> HHHHHHHHSQAGDTLNDVIQDPTRRNKLINDNNLLKGIIMGRDGPVPSSRELIVRPDTLRAIINNRATIETTTMEAEFTETLMESNYNSASVKVSAPFITANSEYSESSSFKNTETEKSMYTSSRYLFPQGRIDFTTPDSGFDDVIKLSPQFTSGVQAALAKATGTEKREALQNLFQEYGHVFRTKVHIGGVLSAHTMETFSRSENETEVKQDVKAGLEGAVKGWGGGATAGHGNTQGTITTSQNRKLNVKYIVNGGDYTKIQNTEEWVASTNQSEHWRVIEVT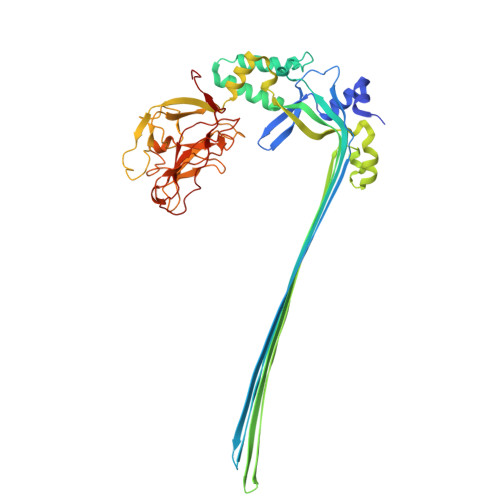EVTAVADLLPQPIRGQVKDLLKPLLGKWVDVEKVPGLESLPVSVYRPKGAIPAGWFWLGDTADASKALLVKPTLPARSGRNPALTSLHQGSGMTEQPFVDLPQYQYLSTYFGSFAHDTPPGSTLRGLRPDHVLPGRYEMHGDTISTAVYVTRPVDVPFPEDECFDLKSLVRVKLPGSGNPPKPRSALKKSMVLFDSGEK> GPLGSMLKDVLTSELAAQVRDAFDDDRDAETFLLRLERYGEDLWESLRAVYGDQVRALPGRLLEVMLHAYHARPAELRRLDEARLLRPDWLQRPEMVGYVAYTDRFAGTLKGVEERLDYLEGLGVKYLHLMPLLRPREGENDGGYAVQDYRAVRPDLGTMDDLSALARALRGRGISLVLDLVLNHVAREHAWAQKARAGDPKYRAYFHLFPDRRGPDAFEATLPEIFPDFAPGNFSWDEEIGEGEGGWVWTTFNSYQWDLNWANPDVFLEFVDIILYLANRGVEVFRLDAIAFIWKRLGTDCQNQPEVHHLTRALRAAARIVAPAVAFKAEAIVAPADLIHYLGTRAHHGKVSDMAYHNSLMVQLWSS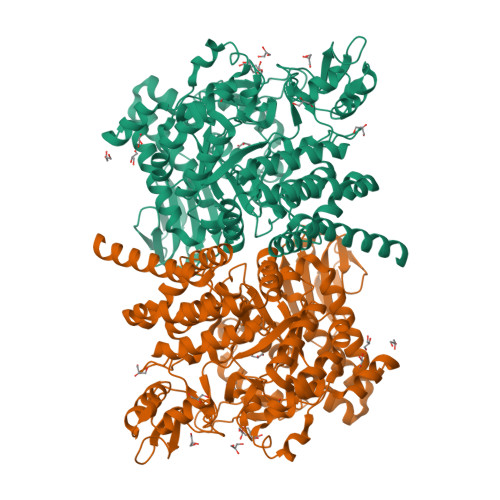LASRNTRLFEEALRAFPPKPTSTTWGLYVRCHDDIGWAISDEDAARAGLNGAAHRHFLSDFYSGQFPGSFARGLVFQYNPVNGDRRISGSAASLAGLEAALETGDPGRIEDAVRRLLLLHTVILGFGGVPLLYMGDELALLNDYAFEDVPEHAPDNRWVHRPQMDWALAERVRQEPSSPAGRVNTGLRHLLRVRRDTPQLHASIESQVLPSPDSRALLLRRDHPLGGMVQVYNFSEETVMLPSHVLRDVLGDHVQDRLSGSAFRLDRPTVRLEGYRALWLTAGEAPA RBM45 is an RNA-binding protein with roles in neural development by regulating RNA splicing. Its dysfunction and aggregation are associated with neurodegenerative diseases such as amyotrophic lateral sclerosis (ALS) and frontotemporal lobar dementia (FTLD). RBM45 consists of three RNA-recognition motif (RRM) domains, two at the N-terminus (RRM1 and RRM2) and one at the C-terminus (RRM3), and a pseudo-RRM domain in the middle. In this work, we identified that the C-terminal RRM domain of human RBM45 (RBM45RRM3) sequence specifically binds GACG sequence RNA and solved the crystal structures of RBM45RRM3 in apo form and in complex with a single-stranded DNA that mimicked the recognized RNA.

To determine the structure of the C-terminal RRM (RRM3) of RBM45, we tried a series of different RBM45 fragments containing RRM3 for crystallization, and finally obtained crystals of a fragment from residue 370 to the C-terminus (hereafter named RBM45RRM3) and resolved its crystal structure at 2.4-Å resolution. There are four RBM45RRM3 molecules per asymmetry unit, containing residues from Gln370 to Arg466 or Glu467. The last nine residues at the C-terminus, including the NLS, are disordered in all four molecules. RBM45RRM3 bears the canonical RRM fold, which is characterized by a βαββαβ topology. The four β-strands form an antiparallel β–sheet in the order of β4–β1–β3–β2, while the two α-helices are located on the same side of the sheet. The exposed side of the β-sheet is predominantly positively charged, indicating a potential RNA binding surface. The overall structure of RBM45RRM3 can be well aligned with the AlphaFold-predicted model with a Cα root-mean-square deviation (RMSD) of 0.42 Å (for 86 residues). The major differences occur in the N-terminal loop, C-terminal loop, and some other loop regions, and these regions also show diversity among the four molecules in the asymmetric unit. The β2–β3 loop of RRM3 is much shorter than those of RRM1 and RRM2, whereas the α2–β4 loop of RRM3 is a little shorter than that of RRM1 and significantly longer than that of RRM2. The most significant difference is that RRM3 has a distinctive N-terminal loop surrounding α1 and touching α2 as well as the α2–β4 loop.

>[4x]MQIQTDVVLPSCKKKAPAETPVKERLFIVFNPHPLPLDVLEDIFCRFGNLIEVYLVSGKNVGYAKYADRISANDAIATLHGKILNGVRLKVMLADSPREESNKRQRTYLEHHHHHH(2S,4R)-1,3-thiazolidine-2,4-diamine | C3 H9 N3 S 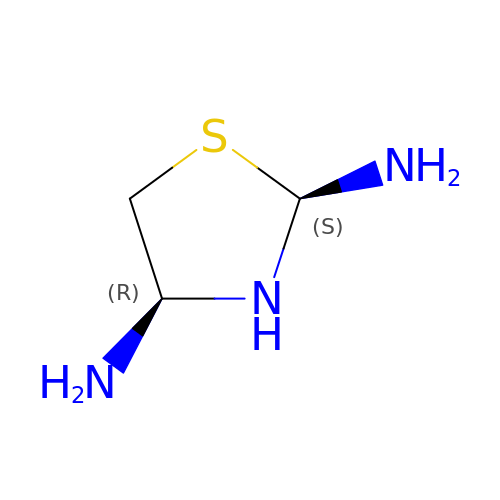| QLBSFPQCZZUQIJ-GBXIJSLDSA-N>[2x]MSDKDSKNTPQVPEKLGLSRRGFLGASAVTGAAVAATALGGAVMTRESWAQAVKESKQKIHVGPGELDDYYGFWSGGHQGEVRVLGVPSMRELMRIPVFNVDSATGWGLTNESRHIMGDSAKFLNGDCHHPHISMTDGKYDGKYLFINDKANSRVARIRLDIMKCDKMITVPNVQAIHGLRLQKVPHTKYVFANAEFIIPHPNDGKVFDLQDENSYTMYNAIDAETMEMAFQVIVDGNLDNTDADYTGRFAAATCYNSEKAFDLGGMMRNERDWVVVFDIHAVEAAVKAGDFITLGDSKTPVLDGRK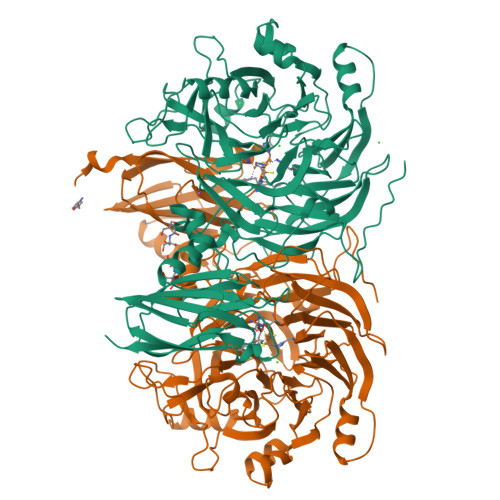KDGKDSKFTRYVPVPKNPHGCNTSSDGKYFIAAGKLSPTCSMIAIDKLPDLFAGKLADPRDVIVGEPELGLGPLATTFDGRGNAYTTLFIDSQVVKWNMEEAVRAYKGEKVNYIKQKLDVHYQPGHLHASLCETNEADGKWLVALSKFSKDRFLPVGPLHPENDQLIDISGDEMKLVHDGPTFAEPHDCIMARRDQIKTKKIWDRNDPFFAPTVEMAKKDGINLDTDNKVIRDGNKVRVYMTSMAPAFGVQEFTVKQGDEVTVTITNIDQIEDVSHGFVVVNHGVSMEISPQQTSSITFVADKPGLHWYYCSWFCHALHMEMVGRMMVEPAWSHPQFEK> ALVIAFIGKNGAVMAGDMREITFEGEKPDREKLEKELYSGSIVTDEEMQKKAEEFGVKITVADCKEKVSERNGVLVGEVSSAEGGVVKKRRLYASAGNFAIAELINTEMTLTSQGKGSNFIAFGNEFTKQVANKCFKDNW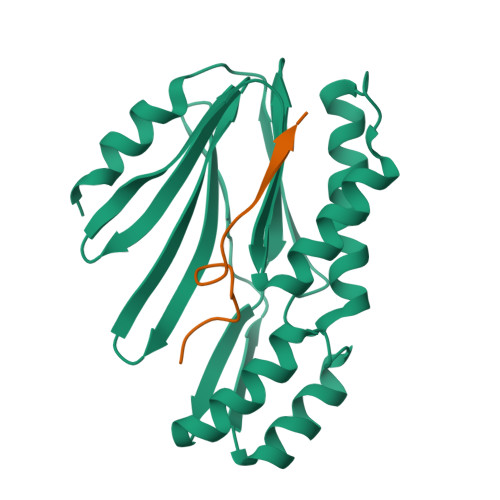TKKSNLQDAVKILILCMETVARKTASVSKQFMIVQTASNADVLKVVEKDRNS;> RELASKDPGAVDAKPLVVEI>GGSDLDQGGEALAPRQVLDLEDLVFTQGSHFMANKRCQLPDGSFRRQRKGYEEVHVPALKPKPFGSEEQLLPVEKLPKYAQAGFEGFKTLNRIQSKLYRAALETDENLLLCAPTGAGKTNVALMCMLREIGKHINMDGTINVDDFKIIYIAPMRSLVQEMVGSFGKRLATYGITVAELTGDHQLCKEEISATQIIVCTPEKWDIITRKGGERTYTQLVRLIILDEIHLLHDDRGPVLEALVARAIRNIEMTQEDVRLIGLSATLPNYEDVATFLRVDPAKGLFYFDNSFRPVPLEQTYVGITEKKAIKRFQIMNEIVYEKIMEHAGKNQVLVFVHSRKETGKTARAIRDMCLEKDTLGLFLREGSASTEVLRTEAEQCKNLELKDLLPYGFAIHHAGMTRVDRTLVEDLFADKHIQVLVSTATLAWGVNLPAHTVIIKGTQVYSPEKGRWTELGALDILQMLGRAGRPQYDTKGEGILITSHGELQYYLSLLNQQLPIESQMVSKLPDMLNAEIVLGNVQNAKDAVNWLGYAYLYIRMLRSPTLYGISHDDLKGDPLLDQRRLDLVHTAALMLDKNNLVKYDKKTGNFQVTELGRIASHYYITNDTVQTYNQLLKPTLSEIELFRVFSLSSEFKNITVREEEKLELQKLLERVPIPVKESIEEPSAKINVLLQAFISQLKLEGFALMADMVYVTQSAGRLMRAIFEIVLNRGWAQLTDKTLNLCKMIDKRMWQSMCPLRQFRKLPEEVVKKIEKKNFPFERLYDLNHNEIGELIRMPKMGKTIHKYVHLFPKLELSVHLQPITRSTLKVELTITPDFQWDEKVHGSSEAFWILVEDVDSEVILHHEYFLLKAKYAQDEHLITFFVPVFEPLPPQYFIRVVSDRWLSCETQLPVSFRHLILPEKYPPPTELLDLQPLPVSALRNSAFESLYQDKFPFFNPIQTQVFNTVYNSDDNVFVGAPTGSGKTICAEFAILRMLLQSSEGRCVYITPMEALAEQVYMDWYEKFQDRLNKKVVLLTGETSTDLKLLGKGNIIISTPEKWDILSRRWKQRKNVQNINLFVVDEVHLIGGENGPVLEVICSRMRYISSQIERPIRIVALSSSLSNAKDVAHWLGCSATSTFNFHPNVRPVPLELHIQGFNISHTQTRLLSMAKPVYHAITKHSPKKPVIVFVPSRKQTRLTAIDILTTCAADIQRQRFLHCTEKDLIPYLEKLSDSTLKETLLNGVGYLHEGLSPMERRLVEQLFSSGAIQVVVASRSLCWGMNVAAHLVIIMDTQYYNGKIHAYVDYPIYDVLQMVGHANRPLQDDEGRCVIMCQGSKKDFFKKFLYEPLPVESHLDHCMHDHFNAEIVTKTIENKQDAVDYLTWTFLYRRMTQNPNYYNLQGISHRHLSDHLSELVEQTLSDLEQSKCISIEDEMDVAPLNLGMIAAYYYINYTTIELFSMSLNAKTKVRGLIEIISNAAEYENIPIRHHEDNLLRQLAQKVPHKLNNPKFNDPHVKTNLLLQAHLSRMQLSAELQSDTEEILSKAIRLIQACVDVLSSNGWLSP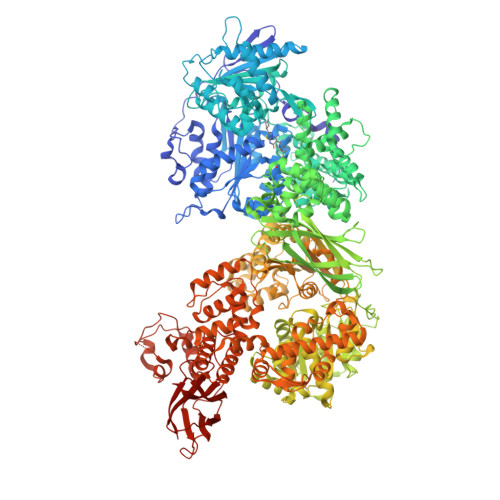ALAAMELAQMVTQAMWSKDSYLKQLPHFTSEHIKRCTDKGVESVFDIMEMEDEERNALLQLTDSQIADVARFCNRYPNIELSYEVVDKDSIRSGGPVVVLVQLEREEEVTGPVIAPLFPQKREEGWWVVIGDAKSNSLISIKRLTLQQKAKVKLDFVAPATGAHNYTLYFMSDAYMGCDQEYKFSVDVKEA[2x]> YSA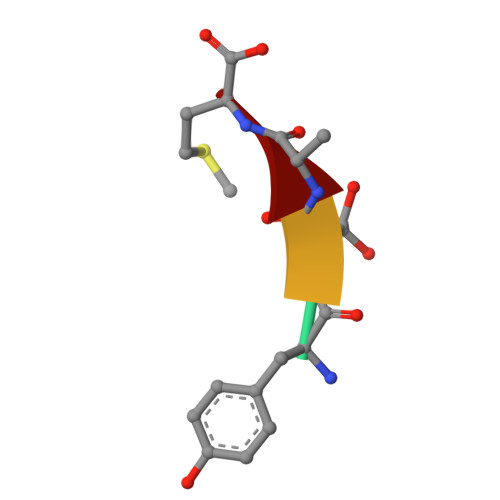M1,2-oxazole-5-carboxamide | C4 H4 N2 O2 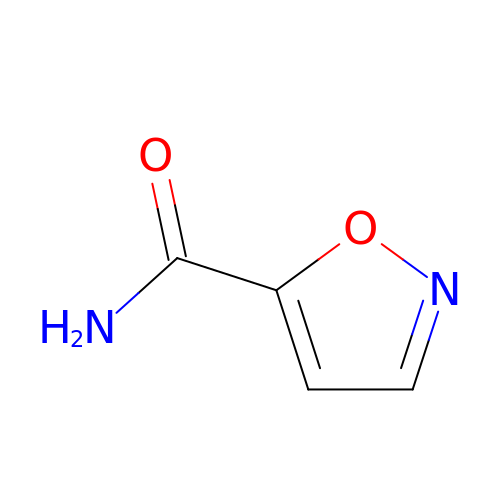| DSIBSRXKQRYPJP-UHFFFAOYSA-N> GSGEADMDFLRNLFSQTLSLGSQKERLLDELTLEGVARYMQSERCRRVICLVGAGISTSAGIPDFRSPSTGLYDNLEKYHLPYPEAIFEISYFKKHPEPFFALAKELYPGQFKPTICHYFMRLLKDKGLLLRCYTQNIDTLERIAGLEQEDLVEAHGTFYTSHCVSASCRHEYPLSWMKEKIFSEVTPKCEDCQSLVKPDIVFFGESLPARFFSCMQSDFLKVDLLLVMGTSLQVQPFASLISK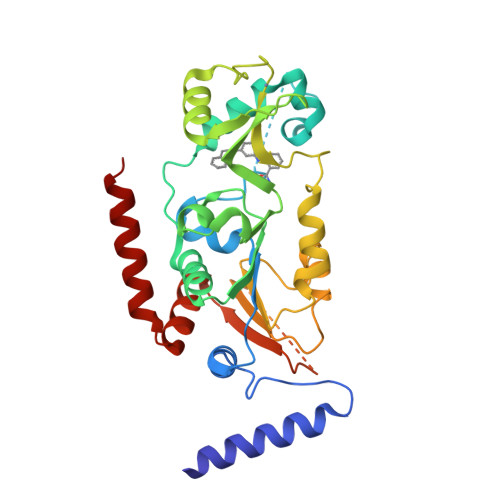APLSTPRLLINKEKAGQSDPFLGMIMGLGGGMDLGETPFDDIATFDSKKAYRDVAWLGECDQGCLALAELLGWKKELEDLVRREHASIDAQS>PYWEIFTPENAFTPDDKEQLSEAITSIYVDYVNLPRFYVVVLFKDMPKETMYVGGKANNNFVRIRLDHIA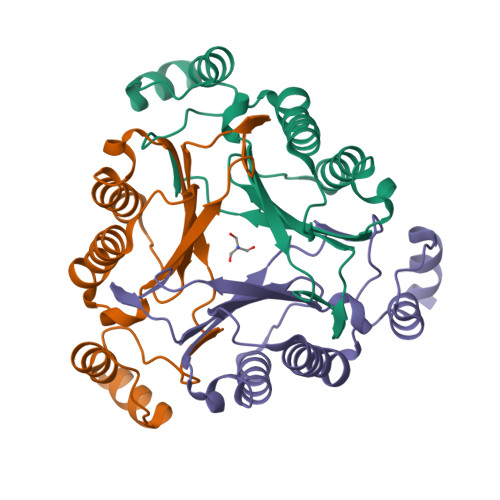RQMETAEVRALMMTVAEEKLAPFIKERGYDWEIHIAETPMDLWRTQGLVPPPPESDMEKLWAKENRPIPYDVAASKLAAALE[3x]>[2x]AECSVDIQGNDQMQF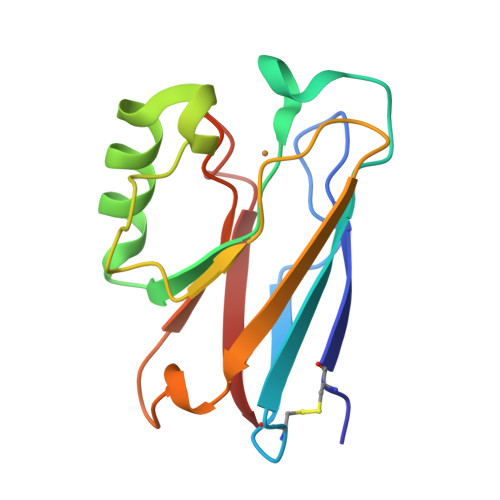NTNAITVDRSCKQFTVNLSHPGNLPKNVMGHNWVLSTAADMQGVVTDGMASGLDKDYLKPDDSRVIAHTKLIGSGEKDSVTFDVSKLKEGEQYMFFCTFPGHSALMKGTLTLK> HMVDSDDDDLVGVPVSPKVPLRTMTPRLARDMSFLIKDKGGLEGMYYSRRRHRILDIYLEKEEGIIPDWHNYTHGPGIRFPKCPGWLWKLVPVDHPQEEQNDEANYLLHP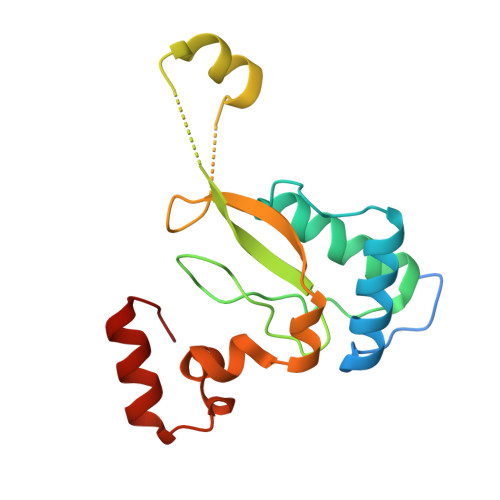AQVSKHDDPHGETLVWRFDPMLAHEYVAFKKYPEEFGYQSGLPEDVWKAKLKARGIPFN>MLYKEPEDGEKIKFDKGKWIVPNKPVILYIEGDGIGPEITNAAIKVINKAVERAYGSSREIKWLEVYAGEKAEKLVNDRFPKETQEMLLKYRVVLKGPLETPIGKGWKSVNVAIRLMLDLYANIRPVKYIEGLESPLKHPEKVDMIIFRENTDDLYRGIEYPFNSEEAKKIRDFLRKELKVEIEDDTGIGIKVMSKYKTQRITRLAIQYAIEHKRKKVTIMHKGNVMKYTEGAFREWAYEVALKEYRDFIVTEEEINQGKPDQGKIILNDRIADNMFQQIIIRPEEYDIILAPNVNGDYISDAAGALIGNIGMLGGANIGDEGGMFEAIHGTAPKYAGKNVANPTGIIKAGELMLRWMGWNEAADLIEKAINMAIRDKKVTQDIARFMG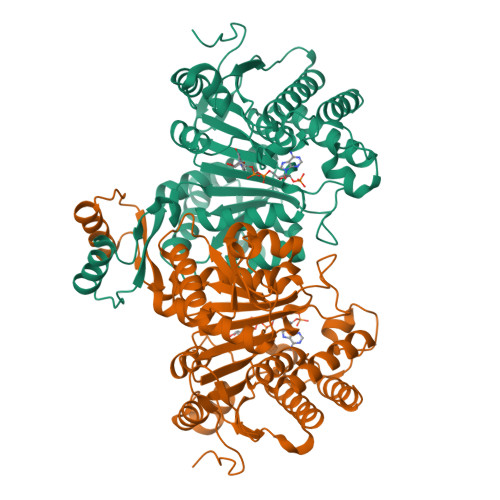VKALGTKEYADELIKIMDTI[2x]>TQFKEIEKTTDFKNHSLPLARIKKIMKADEDVRMISAEAPVVFARACEMFILELTLRSWNHTEENKRRTLQKNDI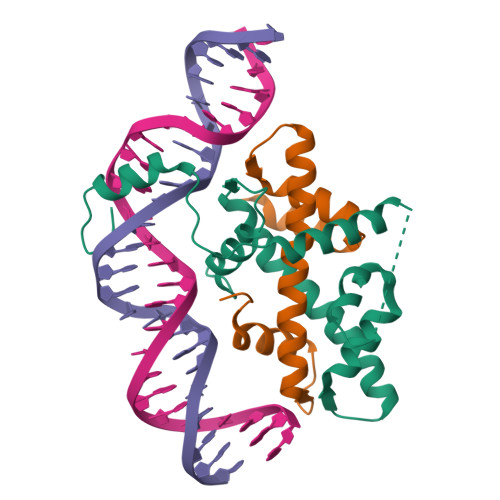AAAVTRTDIFDFLVDIVPRGSGSGSGSGSGSDPASQMITVTQLSPMDREARVLRYREKRKTRKFEKTIRYASRKAYAEIRPRVNGRFAKREIEAEEQGF[4x];>SPREQDRFLPIANVSRIMKKALPANAKISKDAKETMQECVSEFISFVTGEASDKCQKEKRKTINGDDLLWAMTTLGFEDYVEPLKVYLQRFREIEGE[4x]> SVLIPSHAQGELTGRGHKWLEGDSLRTHLTRVEGWVWKNRLLALAMVTVV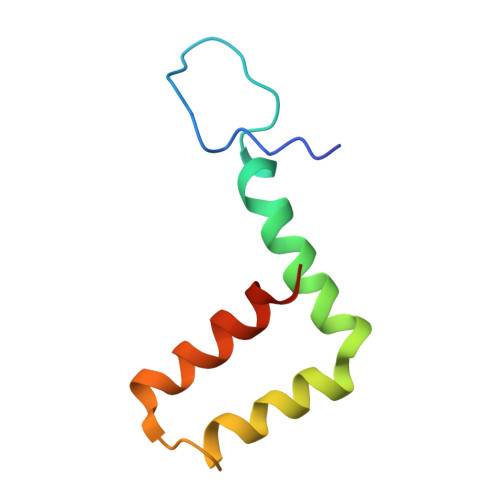WLTLESVVTRVAVLVVLLCLAPVYA>[2x]SAKGYVGDPSDEYYMVTFLSGIDYWKYCFEGFEDAAKAIGVTAKYTGQTDTDVSGQVAVLEQVIAQKPKGIAVTAVNSTALADTINSAIEQGISVVCFDSDSPTSNRSAYLGTGNYAAGQKAAEFLVPLVNYKGKIAVLYTVGAENSESRVQGFEDWCKQNAPEVSLVKVNDAGDTTVAADNLAAALQANDDIVGVFCVDGVAGTAGPTAVAESKKDLR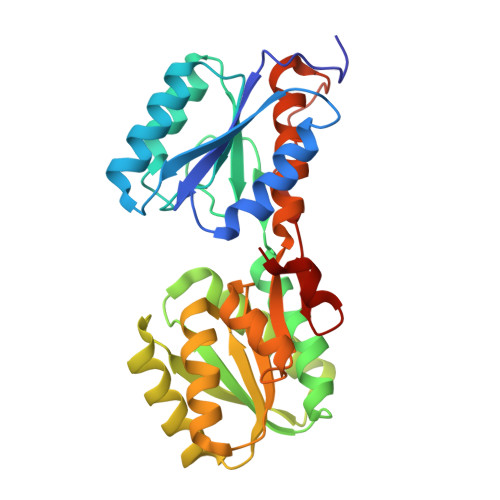VLAFDVDVTVLDKVKSGEIDGTVAQGMYNMGYWSLMMLYTEANGLSSKALPGNLDTGVVIVTKDNVDEYYPKK(6-METHYL-3,4-DIHYDRO-2H-CHROMEN-2-YL)METHYLPHOSPHINATE | C11 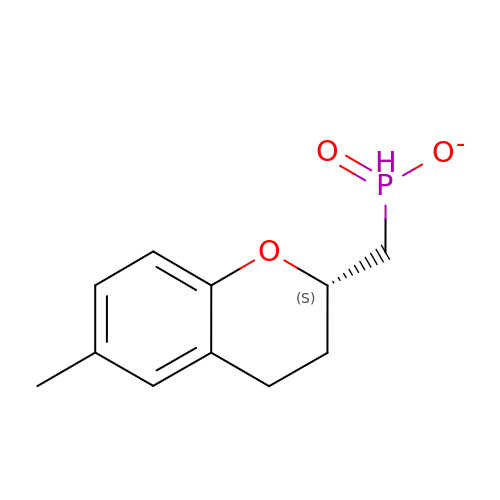H14 O3 P | QTHZTDVLJRQOGF-JTQLQIEISA-M> MELLFLGTGAGIPAKARNVTSVALKLLEERRSVWLFDCGEATQHQMLHTTIKPRKIEKIFITHMHGDHVYGLPGLLGSRSFQGG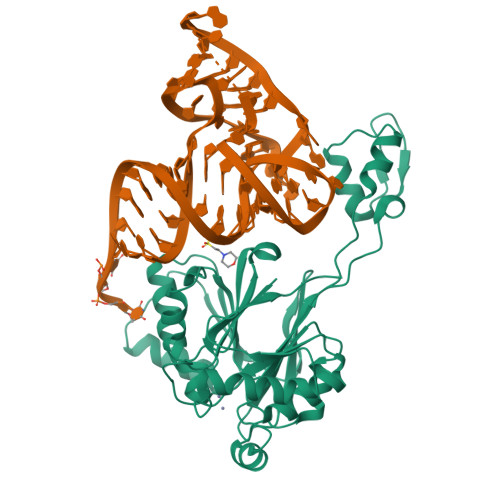EDELTVYGPKGIKAFIETSLAVTKTHLTYPLAIQEIEEGIVFEDDQFIVTAVSVIHGVEAFGYRVQEKDVPGSLKADVLKEMNIPPGPVYQKIKKGETVTLEDGRIINGNDFLEPPKKGRSVVFSGDTRVSDKLKELARDCDVMVHEATFAKEDRKLAYDYYHSTTEQAAVTAKEARAKQLILTHISARYQGDASLELQKEAVDVFPNSVAAYDFLEVNVPRGKLAAALEHHHHHH>GSHMGHWSQGLKISMQDPKMQVYKDEQVVVIKDKYPKARYHWLVLPWTSISSLKAVAREHLELLKHMHTVGEKVIVDFAGSSKLRFRLGYHAIPSMSHVHLHGISQDFDSPCLKNKKHWNSFNTEYF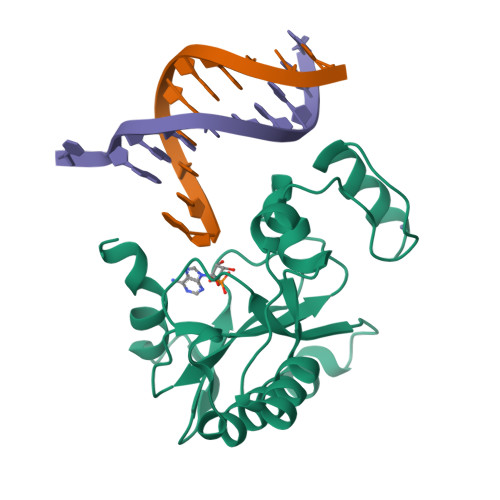LESQAVIEMVQEAGRVTVRDGMPELLKLPLRCHECQQLLPSIPQLKEHLRKHWTQ[2x]Cytosolic phosphoenolpyruvate carboxykinase (PCK1) is a rate-limiting enzyme that catalyzes the reversible conversion of oxaloacetic acid (OAA) into phosphoenolpyruvate (PEP) providing metabolites for several metabolic pathways. We have recently reported that PCK1 activity and stability are subject to a strong posttranslational control by acetylation, phosphorylation, and ubiquitination in response to cell energy input. Thus, the ability of cytosolic phosphoenolpyruvate (PCK1) to perform its reverse reaction (from PEP to OAA) depends on its acetylation level on conserved residues close to the active site. By applying several biophysical and biochemical approaches, we have found that acetyl-CoA promotes the self-acetylation of PCK1, which occurs in the absence of a lysine acetyltransferase.

Analysis of the crystal structure of PCK1 revealed that chemically acetylated lysines were not localized in a specific region of the enzyme, but interestingly, we found acetylation of two lysines inside the active site, K244 and K290, with essential catalytic functions. To analyze the consequences of acetylation of these sites on the kinetic properties of PCK1, we used a previously described method to generate site-specific acetylated PCK1 variants at positions 244 (K244AcK) and 290 (K290AcK) in Escherichia coli ΔCobB. In both cases, acetylation of either K244 or K290 resulted in an enzyme with residual activity (≤1% of controls) under saturated substrate conditions. To gain insight into the consequences of acetylation on K244 and the mechanism of chemical acetylation we crystalized the PCK1 K244AcK variant and PCK1 WT in the presence of acetyl-CoA. However, we were unable to obtain a complex between PCK1 and acetyl-CoA. On the contrary, we were successful in obtaining the crystal structure of PCK1 K244AcK. The structure showed that acetylation on K244 prevents the coordination of Mn2+ with this residue, but interestingly the acetyl group of K244 establishes a hydrogen bond with Arg87 in the R-loop, which is essential for catalysis. These results indicate that acetylation on K244 affects the Mn2+ coordination and also the interaction and synchronization of two essential loops for PCK1 catalysis, leading to PCK1 inactivation. During catalysis, K244 is essential for the coordination of the manganese directly bound to OAA. According to this, site-specific acetylation of K244 prevented manganese coordination and established a hydrogen bond with another catalytic residue, R87, which explained the low activity observed for the enzyme.

> MPPQLHNGLDFSAKVIQGSLDSLPQEVRKFVEGNAQLCQPEYIHICDGSEEEYGRLLAHMQEEGVIRKLKKYDNCWLALTDPRDVARIESKTVIITQEQRDTVPIPKSGQSQLGRWMSEEDFEKAFNARFPGCMKGRTMYVIPFSMGPLGSPLAKIGIELTDSPYVVASMRIMTRMGTSVLEALGDGEFIKCLHSVGCPLPLKKPLVNNWACNPELTLIAHLPDRREIISFGSGYGGNSLLGKKCFALRIASRLAKEEGWLAEHMLILGITNPEGKKKYLAAAFPSACGKTNLAMMNPTLPGWKVECVGDDIAWMKFDAQGNLRAINPENGFFGVAPGTSVKTNPNAIKTIQKNTIFTNVAETSDGGVYWEGIDEPLAPGVTITSWKNKEWRPQDEEPCAHPNSRFCTPASQCPIIDPAWESPEGVPIEGIIFGGRRPAGVPLVYEALSWQHGVFVGAAMRSEATAAAEHKGKVIMHDPFAMRPFFGYNFGKYLAHWLSMAHRPAAKLPKIFHVNWFRKDKNGKFLWPGFGENSRVLEWMFGRIEGEDSAKLTPIGYVPKEDALNLKGLGDVNVEELFGISKEFWEKEVEEIDKYLEDQVNADLPYEIERELRALKQRISQM>MAKKTSSGSETPDLTVATRTGSKDLPIRNIPGNYGLPIVGPIKDRWDYFYDQGAEEFFKSRIRKYNSTVYRVNMPPGAFIAENPQVVALLDGKSFPVLFDVDKVEKKDLLTGTYMPSTELTGGYRILSYLDPSEPKHEKLKNLLFFLLKSSRNRIFPEFQATYSELFDSLEKELSLKGKADFGGSSDGTAFNFLARAFYGTNPADTKLKADAPGLITKWVLFNLHPLLSIGLPRVIEEPLIHTFSLPPALVKSDYQRLYEFFLESAGEILVEADKLGISREEATHNLLFATCFNTWGGMKILFPNMVKRIGRAGHQVHNRLAEEIRSVIKSNGGELTMGAIEKMELTKSVVY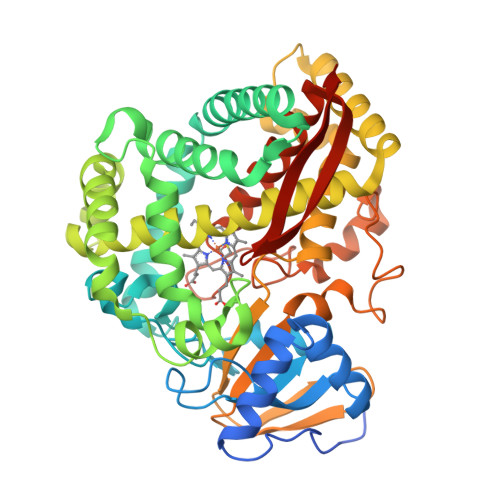ECLRFEPPVTAQYGRAKKDLVIESHDAAFKVKAGEMLYGYQPLATRDPKIFDRADEFVPERFVGEEGEKLLRHVLWSNGPETETPTVGNKQCAGKDFVVLVARLFVIEIFRRYDSFDIEVGTSPLGSSVNFSSLRKASFHHHH[2x]> MIFPKQYPIINFTTAGATVQSYTNFIRAVRGRLTTGADVRHEIPVLPNRVGLPINQRFILVELSNHAELSVTLALDVTNA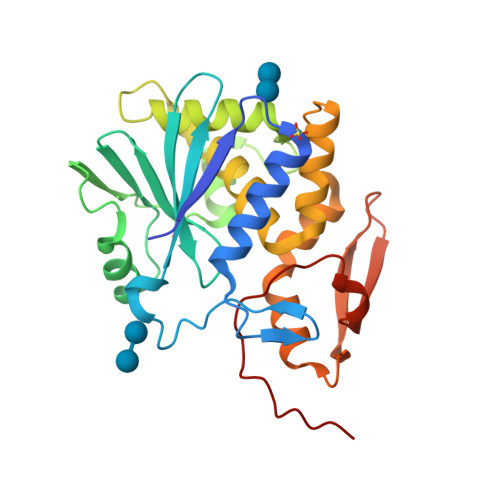YVVGYRAGNSAYFFHPDNQEDAEAITHLFTDVQNRYTFAFGGNYDRLEQLAGNLREDIELGNGPLEEAISALYYYSTGGTQLPTLARSFIICIQMISEAARFQYIEGEMRTRIRYNRRSAPDPSVITLENSWGRLSTAIQESNQGAFASPIQLQRRNGSKFSVYDVSILIPIIALMVYRCAPPPSSQF>[2x]MGRGSHHHHHHGMAMNIKELSLHELCEELKTPAWNVPLTFVGDVGGTSARMGFVREGKNDSVHACVTRYSMKRKDITELIEFFNEIIELMPASVIKRVKAGVINVPGPVTGGAVGGPFNNLKGIARLSDYPKALFPPGRSAILNDLEAGGFGVLA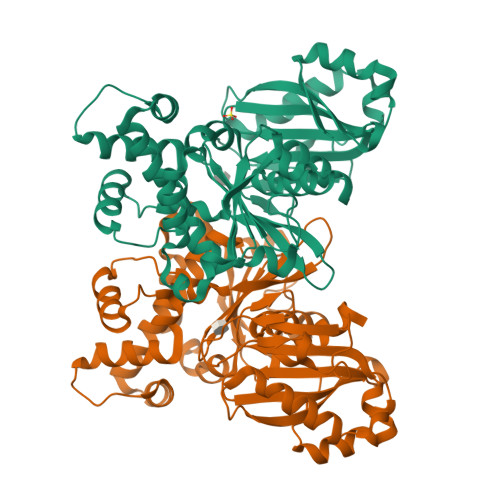VSDAHVFSEYFGVMWEGTQWRTCEQEPAGSVIGRGRCLVLAPGTGLGSSLIYYNPMNQQHIVVPLELGSQTIPMRKDIDYIQTLHAELKLLPNYENMVSGAGLEFHYRQVVRGSRPPCSAGEIAKLASEGDANACKAMKKYHEYLMRVGSEASMALLPLTIVLVGDNIVNNAFFYRNPQNLKEMHREALNHEMERLGFQSRVTYLRQKKLLNLNLMGCYRCGLDLS>MQTEHVILLNAQGVPTGTLEKYAAHTADTRLHLAFSSWLFNAKGQLLVTRRALSKKAWPGVWTNSVCGHPQLGESNEDAVIRRCRYELGVEITPPESIYPDFRYRATDPSGIVENEVCPVFAARTTSALQI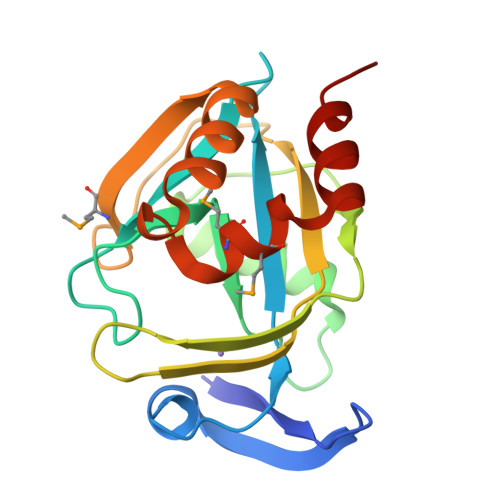NDDEVMDYQWCDLADVLHGIDATPWAFSPWMVMQATNREARKRLSAFTQLK[2x]4-[(2-phenylimidazo[1,2-a]pyrazin-3-yl)amino]benzene-1,2-dicarboxylic 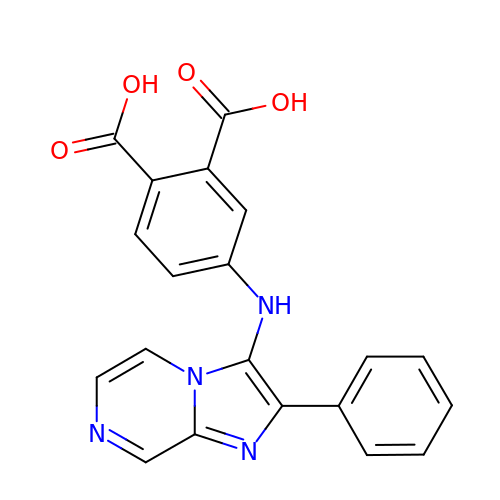acid | C20 H14 N4 O4 | DQITWSHGMZMNEP-UHFFFAOYSA-N We identify Atlas virus—an intact retrovirus-like EVE in the human hookworm Ancylostoma ceylanicum, with an envelope protein genetically related to GN-GC glycoproteins from the family Phenuiviridae. GC proteins are class II membrane fusion proteins, with a three-domain β strand architecture also found in alphaviruses, flaviviruses, and Rubella virus but structurally unrelated to class I fusion proteins. Atlas GC has the hallmarks of an active class II membrane fusion protein: a stable trimeric assembly, a putative fusion loop, membrane insertion triggered by low pH with specificity for late endosomal lipid composition, and membrane fusion activity.

A recombinant ectodomain fragment of Atlas GC (polyprotein residues 2330 to 2772) was expressed in Drosophila melanogaster D.mel-2 cells as a secreted protein. (B) Cryo-EM image reconstruction of a soluble ectodomain fragment of Atlas GC at 3.76 Å overall resolution. The structure reveals a three-domain class II membrane fusion protein fold. The structure of the Atlas GC ectodomain fragment is similar to phlebovirus and bandavirus GC structures, specifically the trimeric postfusion GC structures from RVFV, Dabie bandavirus [DABV, formerly SFTS (severe fever with thrombocytopenia syndrome) phlebovirus] and Heartland virus (HRTV). Domain I, a 10-stranded β barrel augmented by a three-stranded sheet, organizes the structure. Two insertions in domain I form the elongated, mostly β-stranded domain II. Domain III has the seven-stranded β-sandwich topology of fibronectin type III (FN3) domains also found in macroglobulin domains, but the hydrophobic core and disulfide bonding pattern of domain III differ from these and other annotated domains from nonviral species. The most notable differences between Atlas virus and phlebovirus GC structures are differences in the disulfide bonding pattern and in the composition of side chains lining the glycerophospholipid (GPL) headgroup binding pocket conserved in arboviral class II fusion proteins. With 30 cysteine residues forming 15 disulfide bonds, Atlas GC contains twice the average abundance of cysteines, more than has been found in any other class II protein. Specifically, the fusion loop is constrained by four disulfide bonds conserved in phleboviruses and bandaviruses, a fifth disulfide specific to Atlas GC (Cys129 to Cys138), a phenylalanine (Phe136) required in phleboviruses and bandaviruses at the apex of the fusion loop for membrane binding and fusion, and two conserved glycines (Gly128 and Gly134) that provide the torsional flexibility necessary for the fusion loop’s tightly folded conformation.

>[3x]CSEVISVTSTEEVCTIQENKETCTFNHATTITLQPLQQQTCLTLNDPEKRPMGMLTVKPDGIKFRCNKKIEFFTRDHQIVSESVHRCHRAGSCHSDECHHVKDTDALPEFSSEANSRPGYTSCSSSCGCITCDGCFFCEPSCLFHRLYAIPTTPTIYSIFYCPSWELEVDAEISLQREDETTTSTIRLLPGRTSTWNNIRFSLIGTIVPQLPILSSAFVTNGRQTSIVKPAYAGQLQSNSVGQLQCPNLEAAKQFECHFSRNLCTCTNALHKVSCTCYDGSVEDHMEALPLPQTSKNFLVFEKDRNIYAKTHVGSALQLHIVAQDLKITTVKHTSHCQVEASDLSGCYSCTSGASLTLSCKSDNGEVLANMKCNEQTHVIRCTESGFINNILLMFDTSEVAADCTAACPGGIVNFTIKGLLAFVNERIISQSYSATDVERNIKGKPIPNPLLGLDSTRTGHHHHHH In bacteria, the recombination mediator proteins RecO and RecR are required to load the RecA recombinase on ssDNA for homologous recombination. RecO is a key recombination mediator protein that has DNA- and RecR-binding capacities. RecO alone promotes DNA annealing, and it stimulates RecA loading on ssDNA when complexed with RecR. To structurally and functionally characterize RecO, we determined the crystal structure of RecO from Campylobacter jejuni (cjRecO) at a 1.8 Å resolution and biochemically assessed its capacity to interact with DNA and a metal ion. cjRecO folds into a curved rod-like structure that consists of an N-terminal domain (NTD), C-terminal domain (CTD), and Zn2+-binding domain (ZnD).

The crystal structure of cjRecO was determined by single-wavelength anomalous diffraction (SAD) phasing and refined to an Rfree value of 20.8% at a 1.8 Å resolution. The cjRecO structure contains all the residues of the cjRecO polypeptide chain (residues 1–204) and takes the shape of a curved rod consisting of five α-helices and eight β-strands. The curved rod-like structure can be divided into three parts: an N-terminal domain (NTD; residues 1–69), a C-terminal domain (CTD; residues 70–134 and 173–204), and a Zn2+-binding domain (ZnD; residues 135–172). The NTD is composed of five β-strands (β1–β5), which fold into a closed barrel defined as an oligonucleotide/oligosaccharide-binding (OB) fold. The hydrophobic interdomain residues combined with the internal residues of each domain form a continuous hydrophobic core that penetrates through the three domains. Despite the extremely low sequence identity, the cjRecO structure folds into a curved rod-like three-domain structure as observed for ecRecO and drRecO but with relatively high root-mean-square deviation (RMSD) values (2.7–3.0 Å for 173–185 Cα atoms). The Zn2+ ion is located at one end of the rod-like cjRecO structure in the coil-rich ZnD and coordinated by two cysteine residues (C141 and C144) from the α3-β6 loop and by one histidine residue (H162) and one cysteine residue (C165) from the β7-β8 loop. Thus, cjRecO uses the CxxC…HxxC motif to coordinate a Zn2+ ion in a pattern similar to the Zn2+-binding CxxC…CxxC motif of drRecO. In the cjRecO structure, the Zn2+ ion tethers the two extended loops of the coil-rich ZnD and thus seems to stabilize the hydrophobic core of cjRecO at one end of the rod-like cjRecO structure. In particular, in the cjRecO structure, the positive patch is limited to NTD and CTD and does not extend to ZnD (left).

> GSAKDPMQGFILHTQKVKDEDLIVYILSSKMLIKAYRFYGLRHSSILSGYKIDFALEENPSFLPRLKDVLHLGFLWIMQRDKMLIWQEFIRLLYRHLKDVEELDSFYFDLLDECVKRFEKQNPKRVIVDAYLKILEFEGRLHKDFFCFACDEKIQNSITLLRAFLPSHSQCALGFEFEEKKLKQFYSSKNCAIFDDEEIENLYHLIKEGL> CCGATGTGTCTGACAAGATTACGCGCAGTTTCTACGGGGTT;> GAGGTGCCGCCAGGCCAGTGAGCCTGGAGAATTCGCGCTTTTTTT;> TTTTTTTTTTTGGGGTCAAGAAAGCGAAATTTTT;> TTTTTAATAGTTTGCGCTGAAAAGCGGTTAGCTCCTTTTTT;> CTACGTGTCCACTATTAAAGATTATAAAAATCAGCCCCCGAA;> ACAAGAGAACCATCACCCTAATCAAGTTTTT;> TTTTTGTTGTTCCAGTTTGGACGAGATA;> TTTTTTCGGTCCTCCGAATGCCATCCGTATTTTT;> CAGAAGTTTTGGTAAACGTTGAAACTCACGTTAT;> CCGCAGTTTAAAAGGCTGTTGAGATCCAGTTCGATAAGGGAA;> GTGGCACTTTTCGGGGAAATGTGCGCGGAACCCCTATTTGTTTATTTTTCTAAATACATTCAAATATGTATCCGCTCATGAGACAATAACCCTGATAAATGCTTCAATAATATTGAAAAAGGAAGAGTATGAGTATTCAACATTTCCGTGTCGCCCTTATTCCCTTTTTTGCGGCATTTTGCCTTCCTGTTTTTGCTC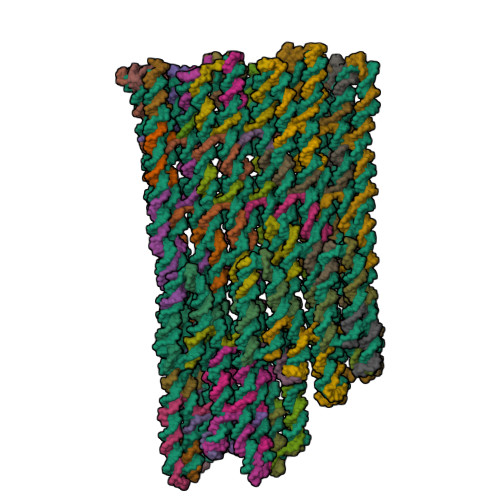ACCCAGAAACGCTGGTGAAAGTAAAAGATGCTGAAGATCAGTTGGGTGCACGAGTGGGTTACATCGAACTGGATCTCAACAGCGGTAAGATCCTTGAGAGTTTTCGCCCCGAAGAACGTTTTCCAATGATGAGCACTTTTAAAGTTCTGCTATGTGGCGCGGTATTATCCCGTATTGACGCCGGGCAAGAGCAACTCGGTCGCCGCATACACTATTCTCAGAATGACTTGGTTGAGTACTCACCAGTCACAGAAAAGCATCTTACGGATGGCATGACAGTAAGAGAATTATGCAGTGCTGCCATAACCATGAGTGATAACACTGCGGCCAACTTACTTCTGACAACGATCGGAGGACCGAAGGAGCTAACCGCTTTTTTGCACAACATGGGGGATCATGTAACTCGCCTTGATCGTTGGGAACCGGAGCTGAATGAAGCCATACCAAACGACGAGCGTGACACCACGATGCCTGTAGCAATGGCAACAACGTTGCGCAAACTATTAACTGGCGAACTACTTACTCTAGCTTCCCGGCAACAATTAATAGACTGGATGGAGGCGGATAAAGTTGCAGGACCACTTCTGCGCTCGGCCCTTCCGGCTGGCTGGTTTATTGCTGATAAATCTGGAGCCGGTGAGCGTGGGTCACGCGGTATCATTGCAGCACTGGGGCCAGATGGTAAGCCCTCCCGTATCGTAGTTATCTACACGACGGGGAGTCAGGCAACTATGGATGAACGAAATAGACAGATCGCTGAGATAGGTGCCTCACTGATTAAGCATTGGTAACTGTCAGACCAAGTTTACTCATATATACTTTAGATTGATTTAAAACTTCATTTTTAATTTAAAAGGATCTAGGTGAAGATCCTTTTTGATAATCTCATGACCAAAATCCCTTAACGTGAGTTTTCGTTCCACTGAGCGTCAGACCCCGTAGAAAAGATCAAAGGATCTTCTTGAGATCCTTTTTTTCTGCGCGTAATCTGCTGCTTGCAAACAAAAAAACCACCGCTACCAGCGGTGGTTTGTTTGCCGGATCAAGAGCTACCAACTCTTTTTCCGAAGGTAACTGGCTTCAGCAGAGCGCAGATACCAAATACTGTTCTTCTAGTGTAGCCGTAGTTAGGCCACCACTTCAAGAACTCTGTAGCACCGCCTACATACCTCGCTCTGCTAATCCTGTTACCAGTGGCTGCTGCCAGTGGCGATAAGTCGTGTCTTACCGGGTTGGACTCAAGACGATAGTTACCGGATAAGGCGCAGCGGTCGGGCTGAACGGGGGGTTCGTGCACACAGCCCAGCTTGGAGCGAACGACCTACACCGAACTGAGATACCTACAGCGTGAGCTATGAGAAAGCGCCACGCTTCCCGAAGGGAGAAAGGCGGACAGGTATCCGGTAAGCGGCAGGGTCGGAACAGGAGAGCGCACGAGGGAGCTTCCAGGGGGAAACGCCTGGTATCTTTATAGTCCTGTCGGGTTTCGCCACCTCTGACTTGAGCGTCGATTTTTGTGATGCTCGTCAGGGGGGCGGAGCCTATGGAAAAACGCCAGCAACGCGGCCTTTTTACGGTTCCTGGCCTTTTGCTGGCCTTTTGCTCACATGTTCTTTCCTGCGTTATCCCCTGATTCTGTGGATAACCGTATTACCGCCTTTGAGTGAGCTGATACCGCTCGCCGCAGCCGAACGACCGAGCGCAGCGAGTCAGTGAGCGAGGAAGCGGAAGAGCGCCCAATACGCAAACCGCCTCTCCCCGCGCGTTGGCCGATTCATTAATGCAGCTGGCACGACAGGTTTCCCGACTGGAAAGCGGGCAGTGAGCGCAACGCAATTAATGTGAGTTAGCTCACTCATTAGGCACCCCAGGCTTTACACTTTATGCTTCCGGCTCGTATGTTGTGTGGAATTGTGAGCGGATAACAATTTCACACAGGAAACAGCTATGACCATGATTACGCCAAGCGCGAATTCTCCAGGCTTAGAATTCGCTCACTGGCCGTCGTTTTACACCATGATTACGCCAAGCGCGAATTCTCCAGGCTTAGAATTCGCTCACTGGCCGTCGTTTTACAACGTCGTGACTGGGAAAACCCTGGCGTTACCCAACTTAATCGCCTTGCAGCACATCCCCCTTTCGCCAGCTGGCGTAATAGCGAAGAGGCCCGCACCGATCGCCCTTCCCAACAGTTGCGCAGCCTGAATGGCGAATGGGACGCGCCCTGTAGCGGCGCATTAAGCGCGGCGGGTGTGGTGGTTACGCGCAGCGTGACCGCTACACTTGCCAGCGCCCTAGCGCCCGCTCCTTTCGCTTTCTTCCCTTCCTTTCTCGCCACGTTCGCCGGCTTTCCCCGTCAAGCTCTAAATCGGGGGCTCCCTTTAGGGTTCCGATTTAGTGCTTTACGGCACCTCGACCCCAAAAAACTTGATTAGGGTGATGGTTCACGTAGTGGGCCATCGCCCTGATAGACGGTTTTTCGCCCTTTGACGTTGGAGTCCACGTTCTTTAATAGTGGACTCTTGTTCCAAACTGGAACAACACTCAACCCTATCTCGGTCTATTCTTTTGATTTATAAGGGATTTTGCCGATTTCGGCCTATTGGTTAAAAAATGAGCTGATTTAACAAAAATTTAACGCGAATTTTAACAAAATATTAACGCTTACAATTTAG;> TTCTGAAACCCGACAGGACTTCAAGTCGGTATCT;> TGGCGTTTCCCCCTGGAAGCTTTTTGTTCTGCGCTACACTACGCCACT;> TAGGGAAGATCCTTTGATCTAAAAAAATATGAGT;> TCTGACGCTCAGTGGAACGATTGCCATAAGCTAGATCCAGT;> TCAAGCTTCATTCAGCTCCGCTCGTCGAAGTTGGCTGCATA;> TCAAGGCGAGTTACATGATCTCTTACCTGCTCAT;> AGAGGTGGCCCTGTTCCGACCTTTCTCAGGCTGTGTCTTGAG;> TTTTTCGTAAAAAGGCCGCGTGCAAAAG;> TTTTTCTTTCTCCCTTCGTTCAGCCCGACTTTTT;> CAGTTATTTTGGTATTGCAAGCAGCATCATGGTGTTCACAAT;> AAGGCCATGCTGGCGTTTTTCCATAGGCGAACATGGAGCGGT;> AATACGGTTCGGTGTAGGTCGACACGACTTTAATGAATCGGC;> AGGCGGTCAACGCGCGGGGAGCGGGAAACCGGAAGAGCTGGC;> CACTCAAGATAACGTATCCGCAAAACGATTCGCGCTTGGCGTAGGGGGA;> CTGCGGCTGAGCAACTGTTTCATTCTAAGCGAATTCTAAGCCATTAAGT;> GCTCGGTGCTTCCTCGCTCACTGTTTTT;> TTTTTACTCGCTGCGCCAGGAACTTTTT;> TTTTTCGCTGCGCCTTATCCGGTAAGAGCGAGGTATGTTTTT;> TCCAACCGCCACTGGGCCTAACTCAGCGCAATCTAAGTTCGCCAGTTTTTTT;> TTGCGTATTGGGCGGCTCACTCCTGGGGGGGCCTCTGGGTAACGTAAAG;> GATTAGCACTATCGTGCACGAACCCCCCGGGAAGCAGAGTTGGTAGCTTTTT;> GGCAGCACGGTAAGTTCGCTCCAAGCTGTAGCTCAAAGCCAG;> TTTTTCTCACATTAATTGCGTTGCCTCTTCCCGTTCGG;> TTTTTCGGTGCTACAGATTCATCCATTAAAA;> ATACGAGCCTGTCGTGCCAGCTGCATATGAAGAACCTTAATCAAACTTG;> TCCACTACCACAGAACAAAAATCGACGCATAAAGATACCAT;> AAATTGTCAGGAAATCCGCCCCCCTGACGAGCATCATCAGGG;> CTGTGTGTGTAAAGGCCCGCTTTCCAGTAGGCGGTATCAGCT;> TTTTTGGCGTAATCATGTGAGTGAGCTAATTTTT;> TTTTTTCTTGATCCGGCTCAAAAAGGATCTTCACCTTTTTT;> TGGTAGCAAGATTTTGGTCATTTTAAATATCTGTCACGGGAG;> TTTTTCGTTGTAAAACGACGGGTTTTCC;> TTTTTAGATCCTTTTAAATAGTTGCCTGATTTTT;> ATGAAGTGAGATTAAAACAAACCACCGCTTACCTTAAGTGGTGTAACAG;> TGTGCTGCCTAAAGGTCTATCCTCCAACGTCAAAGCTCCGAA;> TATTTCGGTTCTTGCGGAAAAGTGGCGCCTGCCGCTTACCGGATACCTGTCCGCTTTTT;> AGTGAGGCCCCAGTGCTGCAATGATAACACCAATGAGACAAC;> GAAAGTTCCGCCGCGCTTAATTGCGCGTGGGGAAATTAACCA;> TTCGCTATACAGGGCGCGTCCTGGCAAGCGAGAAATTTGTTA;> AGGGCGACATTCAGGCTGCGCAATTTTT;> TTTTTCTGTTGGGACAGTCACGATTTTT;> TTTTTCTCCCCGTCGTGTAGATAAGCCAGCCGGAAGTTTTT;> GGCTTACAGATTTACTTTATCTACTGTCTCGTTGTAAACGTTCTTCGTTTTT;> CGCTCACCGGCTCCCATCTGGCACCTATCTACGGCTCTGCTGCGCTGTA;> TTTTTGGAGCGGGCGCTAGGGCGCCATTCGCTCGGTGCTGCCTAAGTCATAG;> TTTTTGGCCGAGCGCAGAAGTGGTCCTGCAATCAGCAATAAACCACTACGAT;> GCTTGACAACCACCACCCGCGTGACCCACTATTAAGGCAGCA;> GCCGGCGTCGGAACCAAGGCGTGGAGAACGGCCAGTGAGCGA;> AACGTGGTGTAGCGGTCACGCGCGCCGCTTACGCCCATAAAG;> AGTAAGTAAGTATAGGATCTCGGTGGTTTCCCTCGTGCGCT;> TGCCGGGTGCTACAGGCATCGAAAAACCGGAGCCC;> ATCGGCACGCAAAAGTAACCCACTCGTGCACCCAA;> TCAAAAGAAAAACACTGATCTTCAGCATCTTTTACTTTCATTTTT;> ATAGGCAATAGGGGTTCCGCGATTTAGATGTTGAA;> ATTCGCGTTGTAAGCGTTAATATTTTTT;> TTTTTTTTGTTAAAGGGTTGAGTTTTTT;> TTTTTAGATGCTTTTCTGTGACTGCTCTTGCCCGGCTTTTT;> CTCAACCAAGTCATTCTGAAATGGTTATTTTTAGA;> AAGTGCCAGCGGATCTTTTTCAATATTAGGTGAGCAATAGAC;> AAAATAAACGAATAGTGTATGATAGCAGAAGCGACACGGAAA;> TTTTTTCAGGGTTATTGTCTCATGACCTAAATTAAATTGGAAGGG;> TTTTTGTCAATACGGGATAATACCCATTGGA;> GCGCCACCGGCGACCGAGTTGGTGAGTAATTCTCTCGCCTCC;> TACTCATAAAATGCAAATCCCACGTGGAAGGGCGATGGCCCACACTAAA;> TAAGGCTGTTATCAGGCGTGGTGTCACGGTTCCCAACGATT;> GGAAGGCACTCTTCACATATTTGAATGTCACATTTTCATTTT;> TTTTTCCAGCGTTTCTGTTGAAGCATTTATTTTT;> TTTTTGGGCGAAAACTCTCAAGGACCCCATGTTGTGT Here we identified Vip3Cb1 and Vip3Cc1, the first Vip3 proteins with broad lepidopteran activity discovered outside of Bt from Paenibacillus strains in the P. popilliae-containing clade, most closely linked to P. dendritiformis. Vip3 proteins, including Vip3Cb1 and Vip3Cc1, are highly conserved in Domains (D) I and II involved in pore formation, with divergence in DIII, IV, and V known to be involved in receptor binding to the gut of the insect host. Vip3Cb1 protoxin and trypsin-processed Vip3Cb1 toxin structures were determined using Cryo-EM, resulting in density maps with an estimated resolution of 2.6 Å and 3.0 Å, respectively. Therefore, structural comparisons of Vip3Cb1 to other Vip3 proteins, including commercial Vip3Aa, are consistent with other results, such as amino acid homology, that all Vip3 proteins share the same mechanism of action, even though these originated from a Paenibacillus strain and not from Bt.

Each dimer pair (monomers A/B, or monomers C/D) is conformationally distinct, with equivalency between monomers A and C and monomers B and D. Domains I (DI) (residues 1–192) and II (residues 202–329) are α-helical, whereas DIII (residues 330–533), DIV (residues 534–675), and DV (residues 676–797) are composed of β-sheets, with homology to carbohydrate binding motifs connected by extended loops. DI of each monomer is composed of two twisted α-helices (α2 and N-terminal α3) connected by a five amino acid loop, allowing α2 to fold back to interact with α3. In the tetramer, DI folds into what could resemble the nose of a spaceship, with the monomers arranged in an A-B-D-C configuration. DII forms the spaceship main body (α1, C-terminal α3, α4-α9), containing a central helix (α8) surrounded by other helices, preceded by the tryptic site (Lysine195) for protoxin activation; however, this site had poor density for modeling (residues 195–202). DIII (β1-β14) forms the spaceship base, ending with a helix (α11) that interacts with DII. From DIII, a linker extends, interacting with N-terminal residues, before starting the extended fins of the spaceship, DIV (β15-β24) and DV (β15-β34). Comparisons of available Vip3 structures, determined by either X-ray protein crystallography, Vip3B2160 (45) or Cryo-EM Vip3Aa16 (43) and Vip3Bc1 (44), revealed that the Vip3Cb1 protoxin has an overall similar quaternary “spaceship” structure with α-helical DI-DIII forming the body and β-sheet DIV-V forming the fins. Activation of the Bt Vip3A protoxin occurs by cleavage between domains DI and DII. The Vip3Cb1 N-terminus has the signature Vip3A signal peptide “ALPSF” motif.

>MHHHHHHHHHHGTETVRFQSKQNNNFSVRALPSFIDVFNGIYGFATGIQDIFNMIFGTDTGDLTLEEVLKNQELLYDISGKLEGISGDLSEIIAQGNLNTELAKELLKIANEQNNVLTDVNNKLNAINSMLHIYLPKITNMLSDVMKQNYALSLQIEYLSKQLQEISDKLDVINLNVLINCTCTEITPAYQRIKYVNEKFDELTLATEKTLRAKQGSEDIIANDTLENLTELTELAKSVTKNDMDSFEFYLHTFHDVLIGNNLFGRSALKTAAELITKDEIKTSGSEIGKVYSFLIVLTCLQAKAFLTLTACRKLLGLSDIDYTNILNQHLNDEKNVFRDNILPTLSNKFSNPNYVKTIGSDNYAKVILEAEPGYALVGFEIINDRIPVLKAYKAKLKQNYQVDHQSLSEIVYLDIDKLFCPKNSEQKYYTKSLTFPDGYVITKITFEKKLNNLRYEATANFYDPSTGDIDLNEKQVESTFLQADYISINVSDDDGVYMPLGVISETFLSPINSFELEVDEKSKILTLTCKSYLREYLLESDLINKETSLIAPPNVFISNIVENWNIEADNLEPWVANNKNAYVDSTGGIEGSKALFTQGDGEFSQFIGDKLKPNTDYIIQYTVKGKPAIYLKNKNTGYTMYEDTNGSSEEFQTIAVNYTSETDPSQTHLVFKSQSGYEAWGDNFIILECKAFETPEGPELIKFDDWISFGTTYIRDDVLTIDPSRGGYFRQSLKLDSYSTYNLSFSFSGLWAKVIIKNSHGVVLFEKVSQQSSYVDISESFTTTSNKEGFFIELTGDSRGGFGSFRDFSMKEKFE[4x]>[2x]VFGG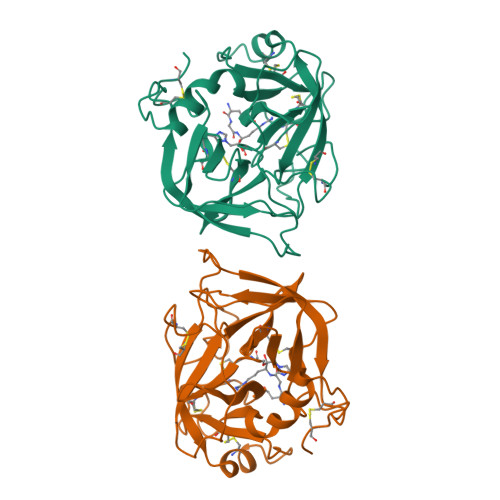DECNINEHRSLVVLFNSNGFLCGGTLINQDWVVTAAHCDSNNFQLLFGVHSKKILNEDEQTRDPKEKFFCPNRKKDDEVDKDIMLIKLDSSVSNSEHIAPLSLPSSPPSVGSVCRIMGWGKTIPTKEIYPDVPHCANINILDHAVCRTAYSWRQVANTTLCAGILQGGRDTCHFDSGGPLICNGIFQGIVSWGGHPCGQPGEPGVYTKVFDYLDWIKSIIAGNKDATCPP> MTVSPVPSPKGRVLIAGATGFIGQFVATASLDAHRPTYILARPGPRSPSKAKIFKALEDKGAIIVYGLINEQEAMEKILK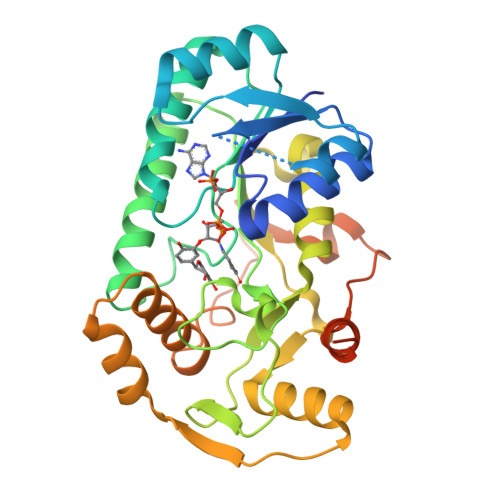EHEIDIVVSTVGGESILDQIALVKAMKAVGTIKRFLPSEFGHDVNRADPVEPGLNMYREKRRVRQLVEESGIPFTYICCNSIASWPYYNNIHPSEVLPPTDFFQIYGDGNVKAYFVAGTDIGKFTMKTVDDVRTLNKSVHFRPSCNCLNINELASVWEKKIGRTLPRVTVTEDDLLAAAGENIIPQSVVAAFTHDIFIKGCQVNFSIDGPEDVEVTTLYPEDSFRTVEECFGEYIVKMEEKQPTADSAIANTGPVVGMRQVTATCA> MALVVQKYGGSSLESAERIRNVAERIVATKKAGNDVVVVCSAMGDTTDELLELAAAVNPVPPAREMDMLLTAGERISNALVAMAIESLGAEAQSFTGSQAGVLTTERHGNARIVDVTPGRVREALDEGKICIVAGFQGVNKETRDVTTLGRGGSDTTAVALAAALNADVCEIYSDVDGVYTADPRIVPNAQKLEKLSFEEMLELAAVGSKILVLRSVEYARAFNVPLRVRSSYSNDPGTLIAGSMEDIPVEEAVLTGVATDKSEAKVTVLGISDKPGEAAKVFRALADAEINIDMVLQNVFSVEDGTTDITFTCPRSDGRRAMEILKKLQVQGNWTNVLYDDQVGKVSLVGAGMKSHPGVTAEFM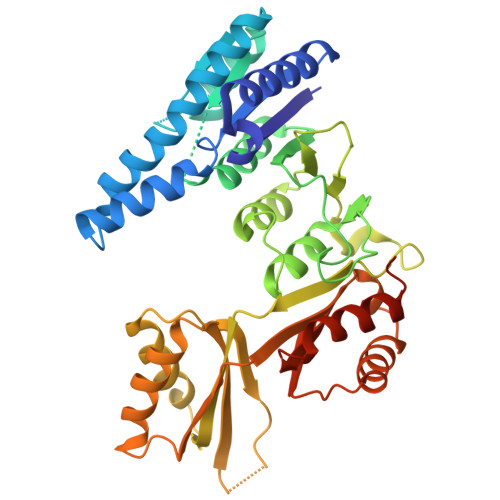EALRDVNVNIELISTSEIRISVLIREDDLDAAARALHEQFQLGGEDEAVVYAGTGR>[7x]MT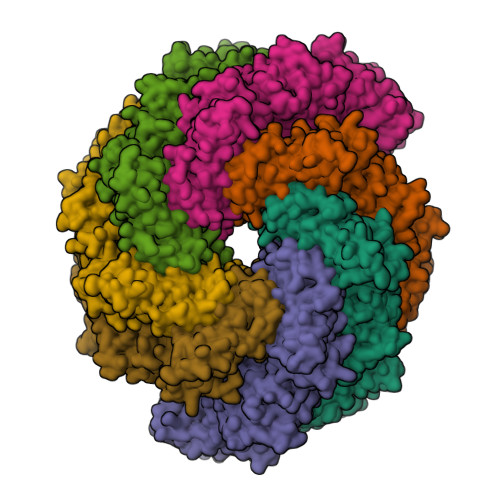DSVQTETTEGKIIINLFAPNLPGSTKEDDLIQKSLRDQLVESIRNSIAYPDTDKFAGLTRFIDESGRNVFFVDGTRGAGKTTFINSVVKSLNSDQDDVKVNIKCLPTIDPTKLPRHEPILVTVTARLNKMVSDKLKGYWASNDYRKQKEQWQNHLAQLQRGLHLLTDKEYKPEYFSDALKLDAQLDYSIGGQDLSEIFEELVKRACEILDCKAILITFDDIDTQFDAGWDVLESIRKFFNSRKLVVVATGDLRLYSQLIRGKQYENYSKTLLEQEKESVRLAERGYMVEHLEQQYLLKLFPVQKRIQLKTMLQLVGEKGKAGKEEIKVKTEPGMQDIDAIDVRQAIGDAVREGLNLREGSDADMYVNELLKQPVRLLMQVLQDFYTKKYHATSVKLDGKQSRNERPNELSVPNLLRNALYGSMLSSIYRAGLNYEQHRFGMDSLCKDIFTYVKQDRDFNTGFYLRPQSESEALRNCSIYLASQVSENCQGSLSKFLQMLLVGCGSVSIFNQFVTELARAENDREKFEQLISEYVAYMSVGRIESASHWANRCCAVVANSPNDEKIGVFLGMVQLNRKSRQHMPGGYKKFNIDTENGLAKAAMASSLSTVASNNLMDFCSVFNLIGAIADISACRCERSAITNAFNKVIAQTTCIVPPWSEAAVRAEMKGSSKSADNDAAVLDVDLDPKDDGVIDESQQDDATEFSDAITKVEQWLKNVNEIEIGIRPSALLIGKVWSRFYFNLNNVADQHKTRLYRNAEHGRMASQSNAAKIMRFNVLAFLHAVLVEESLYHSVSDREYIGEGLRLNPVTSVDEFEKKIKIIGEKLKADNKTWKNTHPLFFLLISCPILHPFIFPVGGINCSVKALNKETSFNKLIDEIVGDKLLSDEEWDYLTKNNDQKTNTRQQIFQNTITSLNSSTIVGASYDKDTPARKTKSPLLGDSEEK> ENLYFQGSEEARE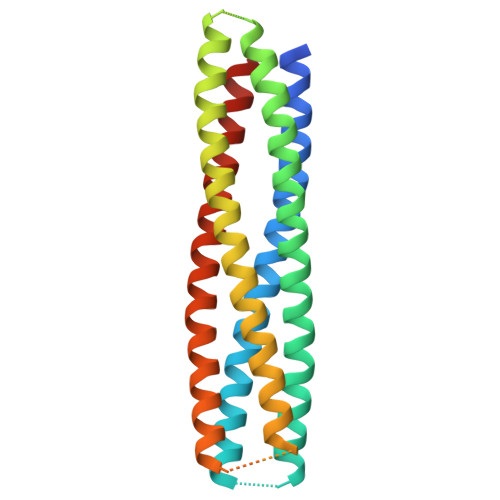VAEEILRLLREHEELLREHERLLKEARELAERLEELARRLEELARRGEKDEEAVRQVEEAAREAERVARELEKSARRLQESIRELRRLLKELRELLRELKKKASEEERKIAEELERIAEEAQRILEETERILRETVRIAQEAVRLLQEARRRAKKGGSGSGENLYFQGGSGSEEIEKLAREIKRAVEELQKALEENERAIRLNKEAARKFEEAVEKFRK> AVSLLDLD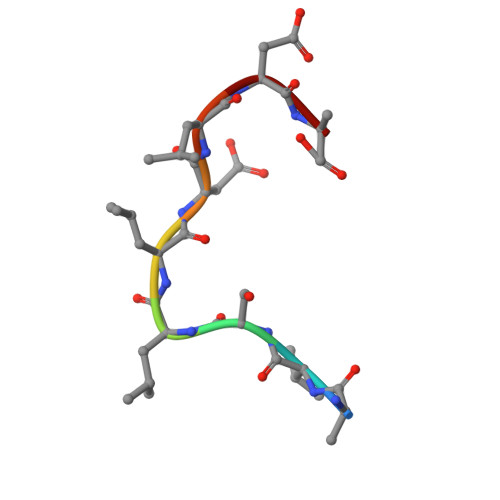A> DNIEDIPLGSSEQDPYDFFTLSDRNVMNSDMKKNIVQWNSRYSYNQLKNKDSLIMFLVEIFRSLFVSNCIDKNIDNVLLSIEEMFIDHYYNPQHSRLKYLIDDVGIFFTKLPITKAFHTYNKKYRITKRLYAPPTFNEVRHILNLAQILSLEEGLDLLTFDADETLYPDGHDFNDEVLASYISCLLKKMNIAIVTAASYNNDAEKYQKRLENLLKYFSKHNIKDGSYKNFYVMGGESNYLFKCNEEATLYSVPENEWRHYKKFVDYDTVQEILNISEKCLEKVIKDFGLCAQIQRKEKSIGLVPNKIPSLNIKNEQKNYMIKYEVLEEAVIRIKKEIIKNKITAPYCAFNGGQDLWVDVGNKAEGLLILQKLLKIQKKKCCHIGDQFLHSGNDFPTRFCSLTLWVSNPQETKACLKSIMHLNIKSFIPEVLYENQ;> KDSLIMFLVEIFRSLFVSNCIDKNIDNVLLSIEEMFIDHYYNPQHSRLKYLIDDVGIFFTKLPITKAFHTYNKKYRITKRLYAPPTFNEVRHILNLAQILSLEEGLDLLTFDADETLYPDGHDFNDEVLASYISCLLKKMNIAIVTAASYNNDAEKYQKRLENLLKYFSKHNIKDGSYKNFYVMGGESNYLFKCNEEATLYSVPENEWRHYKKFVDYDTVQEILNISEKCLEKVIKDFGLCAQIQRKEKSIGLVPNKIPSLNIKNEQKNYMIKYEVLEEAVIRIKKEIIKNKITAPYCAFNGGQDLWVDVGNKAEGLLILQKLLKIQKKKCCHIGDQFLHSGNDFPTRFCSLTLWVSNPQETKACLKSIMHL

Maintaining the optimal nucleotide balance required for normal cell proliferation is controlled by 5′-nucleotidases amongst other processes. These enzymes catalyze the dephosphorylation of ribo- and deoxyribonucleoside monophosphates to their corresponding nucleosides, and also exhibit, in certain cases phosphotransferase activity. All structures adopt a tetrameric assembly displaying a cross-like shape, in agreement with the quaternary solution structure. Each subunit consists of four domains: an “N-Terminal Regulatory Domain” (NTRD, M1 to K59), an “OD” (D60 to T143), a HAD-like Catalytic Domain (CD, F144 to K270 and K371 to Q444) and a C2 cap domain13 (K271 to N370).

With an affinity of 3.8 ± 0.7 mM, ATP is a K-type activator lowering the Km(app) value for IMP tenfold, while kcat(app) remains unchanged. In the tetrameric structure of the ATP-bound wild-type enzyme (PfISN1-ATP), only two ATP molecules located in the two subunits having unstructured NTRDs were observed. The nucleotides bind to a cleft formed by helix α6 from the OD and helices α7 and α16 from the catalytic domain. ATP binds at the very place where the C-terminal loop (LoopL430-Q444) is situated in the PfISN1-Apo structure, implying that this later must leave the cleft upon binding. A π-stacking occurs between H150 and the adenine moiety of ATP, and H150 establishes a bridge between E419 (catalytic domain) and Y129 of the OD. In presence of ATP, no electron density was observed for LoopL430-Q444, suggesting it to be destabilized. Interestingly, in the two subunits showing a structured NTRD but lacking ATP, LoopL430-Q444 stays in the cleft. Upon ATP binding, the enzyme undergoes a conformational change where CD and Cap domains in both β and δ subunits bend, thereby adopting a more closed conformation than that seen for the wild type (whole enzyme RMSD = 1.56 Å). Due to the interactions at interface 1, the ATP induced closure of subunits β and δ forces subunits α and γ to open slightly. Overall, the structures reveal that ATP activates the enzyme by triggering the departure of the LoopL430-Q444 which in turn induces the bending of the subunit thereby increasing the affinity for IMP.>MDALIM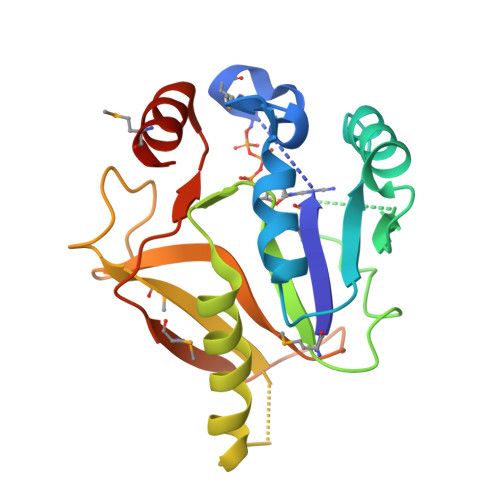AGGKGTRMGGVEKPLIKLCGRCLIDYVVSPLLKSKVNNIFIATSPNTPKTKEYINSAYKDYKNIVVIDTSGKGYIEDLNECIGYFSEPFLVVSSDLINLKSKIINSIVDYFYCIKAKTPDVEALAVMIPKEKYPNPSIDFNGLVPADINVVSPKHGYQKEEIMVIDELIFNINTKDDLKLAEMLLKKDGL[4x]> GRLGFYGYDL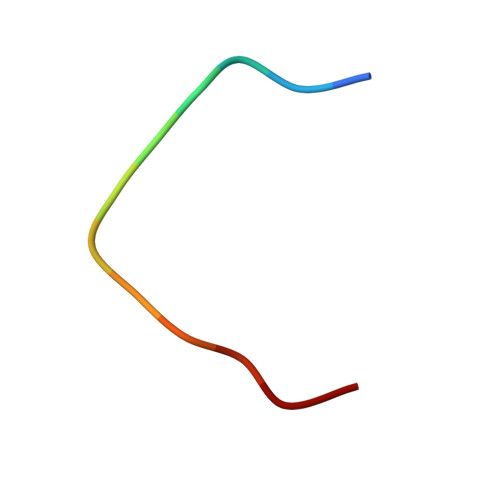QD>TETTSFSITKFSPDQQNLIFQGDGYTTKGKLTLTKAVKSTVGRALYSTPIHIWDRDTGNVANFVTSFTFVIDAPSSYNVADGFTFFIAPVDTKPQTGGGYLGVFNSKEYDKTSQTVAVEFDTFYNAAWDPSNKERHIGIDVNSIKSVNTKSWNLQNGERANVVIAFNA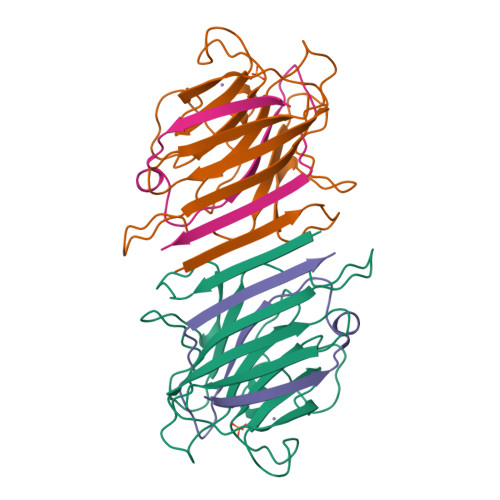ATNVLTVTLTYPN[2x];>VTSYTLNEVVPLKDVVPEWVRIGFSATTGAEFAAQEVHSWSFNSQLGHTSKS[2x]>MTSSEPAHGATPKRSPSEGSADNAALCDALAVEHATIYGYGIVSALSPPGVNFLVADALKQHRHRRDDVIVMLSARGVTAPIAAAGYQLPMQVSSAADAARLAVRMENDGATAWRAVVEHAETADDRVFASTALTES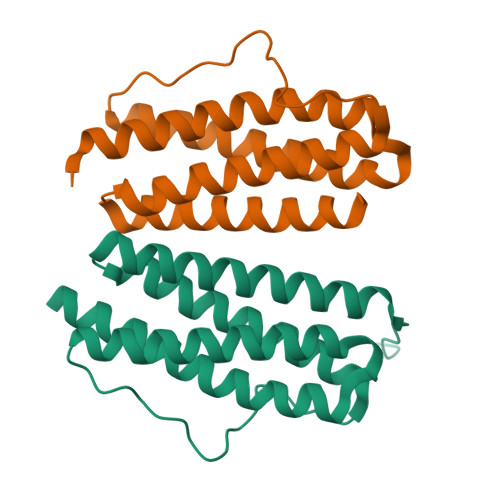AVMATRWNRVLGAWPITAAFPGGDERSHHHHHH[2x]>RFYVKDHRNKAMINLHI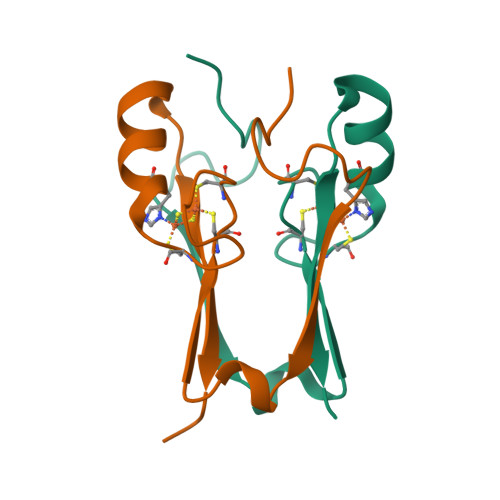QKDNPKIVHAFDMEDLGGKAVYCRCWRSKKFPFCDGAHTKHNEETGDNVGPLIIKKKET[18x]N~2~-{[(1S)-1-carboxy-3-(methylsulfanyl)propyl]carbamoyl}-N~6~-(4-iodobenzoyl)-L-lysine 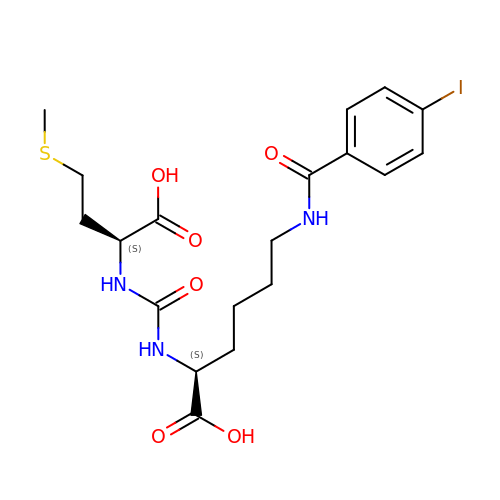| C19 H26 I N3 O6 S | AWPLYTCEHNMVNJ-GJZGRUSLSA-N> MNYTETVAYIHSFPRLAKTGDHRRILTLLHALGNPQQQGRYIHVTGTNGKGSAANAIAHVLEASGLTVGLYTAPFIMRFNERIMIDHEPIPDAALVNAVAFVRAALERLQQQQADFNVTEFEFITALGYWYFRQRQVDVAVIEVGIGGDTDSTNVITPVVSVLTEVALDHQKLLGHTITAIAKHKAGIIKRGIPVVTGNLVPDAAAVVAAKVATTGSQWLRFDRDFSVPKAKLHGWGQRFTYEDQDGRISDLEVPLVGDYQQRNMAIAIQTAKVYAKQTEWPLTPQNIRQGLAASHWPARLEKISDTPLIVIDGAHNPDGINGLITALKQLFSQPITVIAGILADKDYAAMADRLTAAFSTVYLVPVPGTPRALPEAGYEALHEGRLKDSWQEALAASLNDVP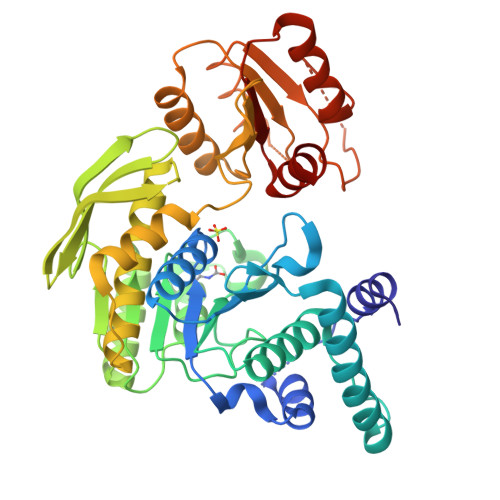DQPIVITGSLYLASAVRQTLLGGKS>[2x]SHRNEAGHGDLHEILHEAVPLDANEREILELKEDAFAQRRREIETRLRAANGKL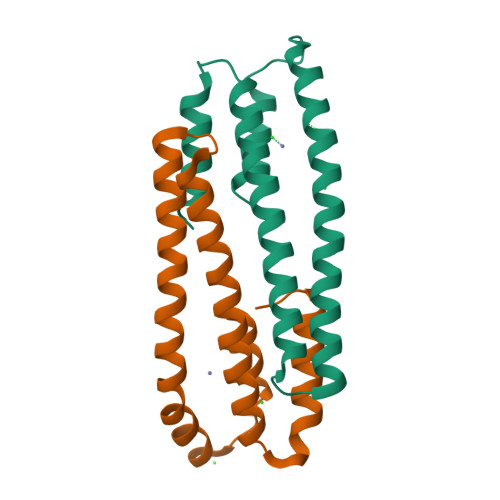ADAIAKNPAWSPEVEAATQEVERAAGDLQRATLVHVFEMRAGLKPEHRPAYDRVLIDALRRGSQ>MVTLAELASDIQSQVKVIDTYLTEHNLPQPTFAPDSPRELPLDANVQRARLLLIEKAMALSNLAIGAADNLRWHCMNNKFDDMTLHFLARYNIFDAVPRDEPISYAELSKKVGLAEHRLRRIMSMAYTQHYFCTPKPGFVAHTSNSAM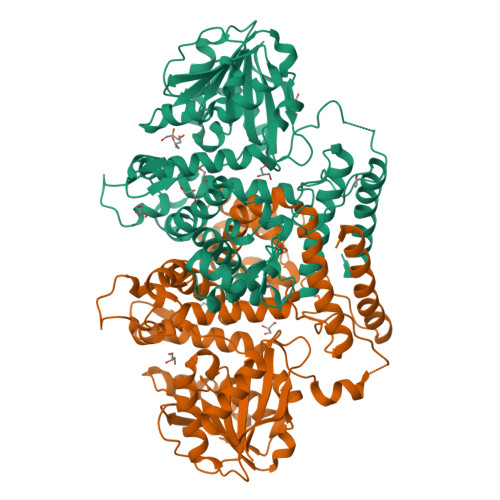AIGDPLALAWILHNIEEVQPWYSNKLVDATMKWGDSIDPKHTGPNLNAKPGEEKLFYEIMEEDDQGEWNGVKGKGFRLWRLYDTDKFFGTGGAIKGTNLLRAFDWGGLGKATVVDIGGITGHLASTVALANPDLTFIVQERNQPWYEKQFYEQLPAELNGRVSYMPHDKYAEQPVKGADVYFMSTVLHKEPDDKAITILRRCVEAMDPNKSRLLTRDIVMDGGDPPAEDAVINGRAINSKEGSYEAGLGPTGVITRLNIGIDFQVLAVVNGFERTREEWVTLFKKADPRFALKGCIQTVGNCAALMEWILEE[2x]> NPVENYIDEVLNEVLVVPNINSSNPTTSNSAPALDAAETGHTSSVQPEDVIETRYVQTSQTRDEMSLESFLGRSGCIHESKLE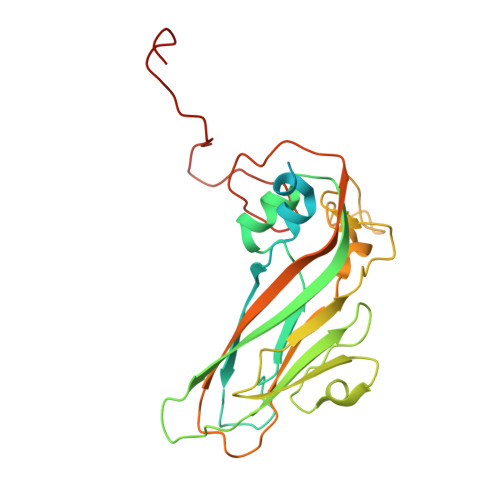VTLANYNKENFTVWAINLQEMAQIRRKFELFTYTRFDSEITLVPCISALSQDIGHITMQYMYVPPGAPVPNSRDDYAWQSGTNASVFWQHGQAYPRFSLPFLSVASAYYMFYDGYDEQDQNYGTANTNNMGSLCSRIVTEKHIHKVHIMTRIYHKAKHVKAWCPRPPRALEYTRAHRTNFKIEDRSIQTAIVTRPIITTAGPSDMY>MSAIRDVMTKFAEQTTMHGVPKVINAKSSMGRLFWSLVCLAAGAMFCLQMSEVLQRYFSYPKKVTVEVVPTPVPFPSISICNMRNLDVHILNTLNRMFIEDDRPFSNINKSEHEFIRAYMKKVAKYAPLFWNYQDEYPEVFQEIFSRTTFSANIDPEVIALAAVQLEGFVVNCHYAGHRCNKTRDFYRFFDPYYFNCFTYKAHEPTDIEDNLSEGIENGWSSILLSGSGMLDKNDEIRMLPGLHEWRSAVSASEGVRVVIHPPSTTPYPFTEGYDVPPGFSASFGIHPRRNIRIGPPHGNCSDKNPFGDGTERYRLMACQKMCMQHYIVETCGCADVGLPKLPLQANISWCRDDDNFPDECMFTASEECLQLLMQLHNRIKCARSIKSKITKNTTAMEACNCFPPCDEVSYDVSYSLSKWPSAGYEGDAAYFDVFGIEKFNERFNKTGTQGKYELFTKYFNVSNREESMKDFARLNVYIADSNVVKTQESEDYTRNQLVSDIGGQLGLWVGISLITLAEVLELIIDLFRLFSKHTYRSVPVIRQSIKYKDKRNGAEMNYDTRYSQSNGGPHARYLHHGHSIPKHPPELPDTSLALEVLFQ[3x]

Here we dissected the structural basis for neuropeptide-gated activity of a neuropeptide-gated DEG/ENaC, FMRFamide-gated sodium channel 1 (FaNaC1) from the annelid worm Malacoceros fuliginosus, using cryo-electron microscopy. We solved high-resolution structures of FaNaC1 alone, with full agonist FMRFa, with partial agonist ASSFVRIa, and with both FMRFa and pore-blocker diminazene, identifying the ligand-binding site and elucidating the conformational changes induced by ligand binding. Each subunit comprises a minimal N terminus and a nonresolved 63-amino acid C terminus facing the intracellular side, two transmembrane segments (TM1 and TM2), and a large extracellular domain. The FaNaC1 structures presented here capture a ligand-free resting state, two ligand-bound desensitized states and a ligand-bound dilated channel state.

Preparations of FaNaC1 alone and with FMRFa (30 μM) yielded 3D reconstructions with a global resolution of 2.7 and 2.5 Å, respectively. For both structures, density could be unambiguously assigned to amino acid sequence based on mostly continuous main chain density and numerous distinctive side chain densities. The 63-amino-acid C-terminal tail was not resolved. To establish how ligand binding induces channel gating, we compared ligand-free and ligand-bound FaNaC1 structures. In both ligand-bound structures, however, the channel pore appears closed, with radii of ~1 Å at the level of G503 and G506 in TM2a (G3′ and G6′ in a TM2 numbering scheme). This is similar to our ligand-free, inactive FaNaC1 structure and is too narrow to pass even mostly dehydrated Na+ ions (~2.3 Å). We also observed a remarkably large conformational change in the β5–β6 loop (residues K200–G218) of the extracellular domain, which flips from a downward orientation in our ligand-free structure to an upward orientation in all ligand-bound structures. This involves, for example, L211 displacing 20 Å and is a notable exception to the otherwise immobile palm/ball domain. Thus, the H297S mutation increases gating efficacy. This suggests that WT resting FaNaC1 channels are energetically primed for opening but cannot do so until ligand binding and extracellular domain rolling releases TM1/TM2a via outward H297 movement.>MIELSLAEALFLILFTGVISMLISRRTGISYVPIFILTGLVIGPLLKLIPRDLAHEIFDFVRVFGLVIILFTEGHNLSWRLLKKNMPTIVTLDTIGLILTALIAGFIFKVVFNSSFLLGFLFGAIIGATDPATLIPLFRQYRVKQDIETVIVTESIFNDPLGIVLTLIAISMLVPGYGGGIFSTLSEKLGIYAGGVIYFLYNVSVSISLGIFLGILGYKFIKRTGIFDFPEIEAFSLSLAFLGFFIGERLDASGYLVATVTGIVLGNYKLLKPRENIRILKRLQRAIEKEVHFNDTLAALATIFIFVLLGAEMNLEVIWSNLGKGLLVALGVMILARPLATLPLLKWWNFREYLFIALEGPRGVVPSALASLPLSLALKYKSPLLTVHWGEIIMATVV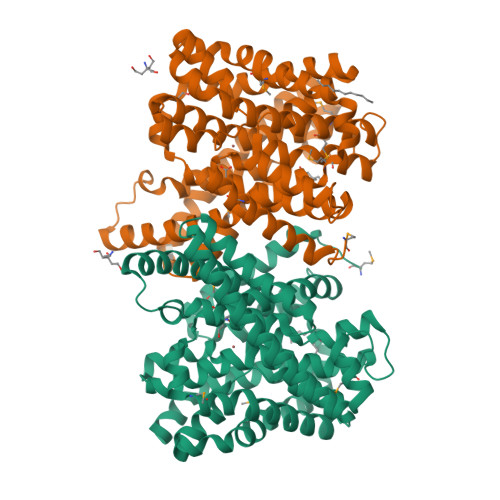ITVLTSVIVETLWIPILKDKLD[2x]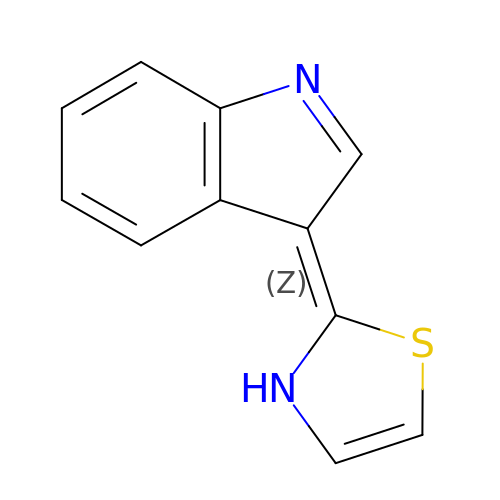(2Z)-2-indol-3-ylidene-3H-1,3-thiazole | C11 H8 N2 S1 | IUBODNCSFJZWGR-PKNBQFBNSA-N>[3x]FVPNKEQTRTVLIFCFHLKKTAAESHRMLVEAFGEQVPTVKTCERWFQRFKSGDFDVDDKEHGKPPKRYE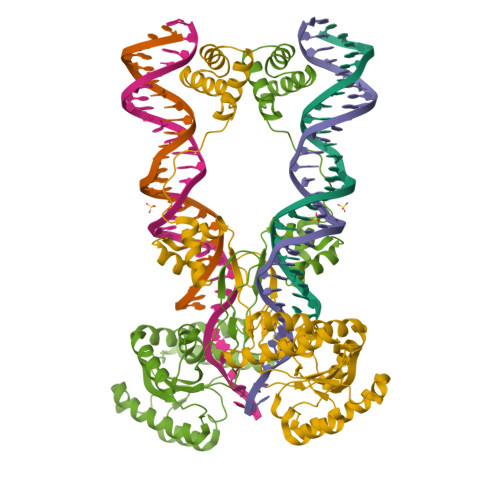DAELQALLDEDDAQTQKQLAEQLEVSQQAVSNRLREMGKIQKVGRWVPHELNERQMERRKNTCEILLSRYKRKSFLHRIVTGDEKWIFFVNPKRKKSYVDPGQPATSTARPNRFGKKTMLCVWWDQSGVIYYELLKPGETVNAARYQQQLINLNRALQRKRPEYQKRQHRVIFLHANAPSHTARAVRDTLETLNWEVLPHAAYSPDLAPSDYHLFASMGHALAEQRFDSYESVKKWLDEWFAAKDDEFYWRGIHKLPERWEKCVASDGKYFE4-chloranyl-2-methyl-5-(methylamino)pyridazin-3-one 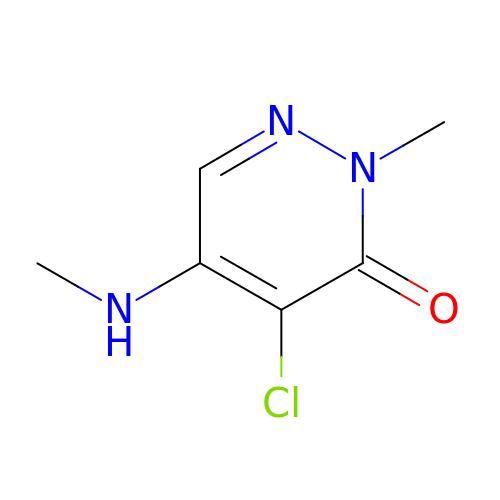| C6 H8 Cl N3 O | ACZYSEPOODWZET-UHFFFAOYSA-N4-fluoranyl-~{N}-[(2~{S})-1-[[4-[(2-methyl-1-oxidanyl-propan-2-yl)sulfamoyl]phenyl]amino]-1-oxidanylidene-3-phenyl-propan-2-yl]benzamide 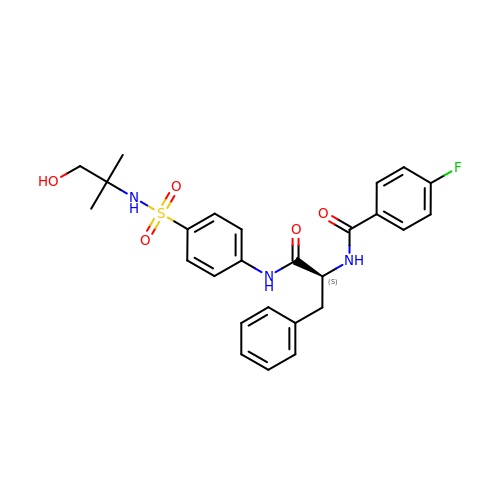| C26 H28 F N3 O5 S | FEWSFPBWIPYPHW-UHFFFAOYSA-N>[8x]MASSTNPITKAKFQSYNYPNMYIRHANFDARIDENVTPEMDSQWELVPGLANSGDGYVSIQSVNYPGYYLRHSNYDLSLEKNDGTSLFAESAT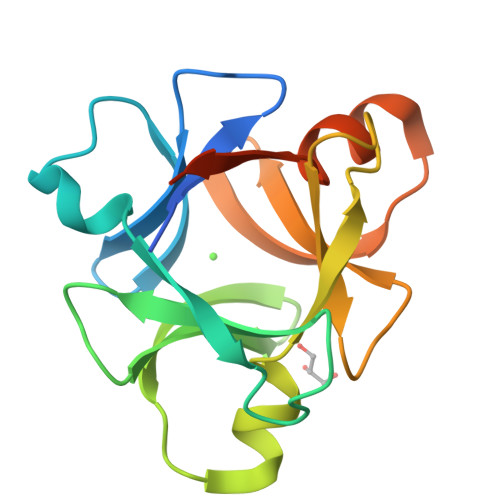FKIVPGLADPSYISFQSYNFPTRYIRHYNYLLRLDEIVTELDRQDATFKIISEDTQLEHHHHHH In this study, we used d(CGTATACG)2, which forms a tetraplex base-pair junction that resembles the DNA–DNA contact structure, as a model target for two alkyl-linked diaminoacridine bis-intercalators, DA4 and DA5. To explore the possibility of targeting inter-DNA duplex structures, we synthesized two acridine-based derivatives, DA4 and DA5, by coupling 9-aminoacridine moieties with hydrocarbon chains of four and five atoms, respectively. Cross-linking of the junction site by the bis-intercalators induced substantial structural changes in the DNA, transforming it from a B-form helical end-to-end junction to an over-wounded side-by-side inter-duplex conformation with A-DNA characteristics and curvature. Furthermore, we have shown that the different topological changes induced by DA4 and DA5 lead to the inhibition of topoisomerase 2 activities, which may account for their antitumor effects.

To understand the structural basis of the binding of DA4 and DA5, we determined the crystal structures of DA4 and DA5 with the d(CGTATACG)2 sequence in the C2221 and P21 space groups, respectively, at a resolution of 1.58 Å. The structure of the DA4–DNA complex features an asymmetric unit with a single duplex intercalated with one DA4 moiety, two Mn2+ ions, and 42 water molecules. In contrast to the unliganded DNA structure, the crystal assembly of the DA4–DNA and DA5–DNA complexes revealed that the duplexes were juxtaposed near terminal CpG sites (C1pG2 and C7*pG8*, respectively), with DA4 and DA5 bis-intercalating into neighboring duplexes. Instead, the intercalation of DA4 and DA5 induced changes in the DNA topology from an end-to-end straight helix to a side-by-side curvature geometry. The four-carbon linker of DA4 adopted a relatively straight conformation, in contrast to the five-carbon linker of DA5, which bent toward the DNA backbone. In the DA4–DNA complex, the two chromophores formed an angle of ∼60° with the horizontal plane of the acridine ring, whereas in the DA5–DNA complex, the angle between the two acridine chromophores was ∼50°. In DA4–DNA complex, three water molecules mediate indirect interactions between two inter-strand cytosine bases and the DA4. In the DA4–DNA complex structure, the straight linker and highly tilted chromophore of DA4 create space for accommodating water. However, the increased distance between the amino group of the linker and the keto group of cytosine leads to indirect and weaker interactions. The sum of roll angles of central five steps was 35.3° and 32.8° for DA4–DNA and DA5–DNA complex structures, respectively, suggesting a sharp curvature in the backbone upon compound intercalation.

>[2x]CGTATACG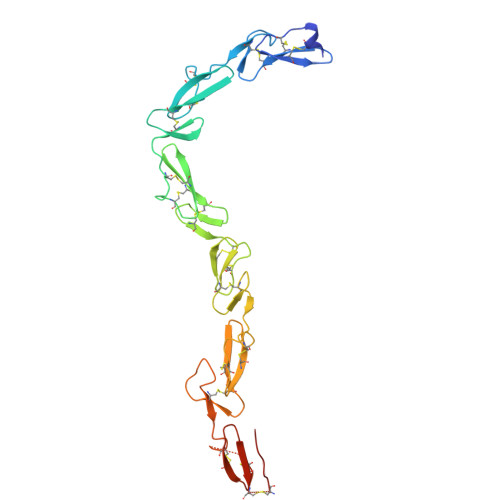> AGYDFCSERHNCMENSICRNLNDRAVCSCRDGFRALREDNAYCEDIDECAEGRHYCRENTMCVNTPGSFMCICKTGYIRIDDYSCTEHDECITNQHNCDENALCFNTVGGHNCVCKPGYTGNGTTCKAFCKDGCRNGGACIAANVCACPQGFTGPSCETDIDECSDGFVQCDSRANCINLPGWYHCECRDGYHDNGMFSPSGESCEDIDECGTGRHSCANDTICFNLDGGYDCRCPHGKNCTGHHHHHH>[6x]MGSSWSHPQFEKSSGMNNIDLRVYSFIDSLQPQLASYLATSSQGFLPVPGDACLWIEVAPGMAVHRLSDIALKATNVRLGEQVVERAFGSMEI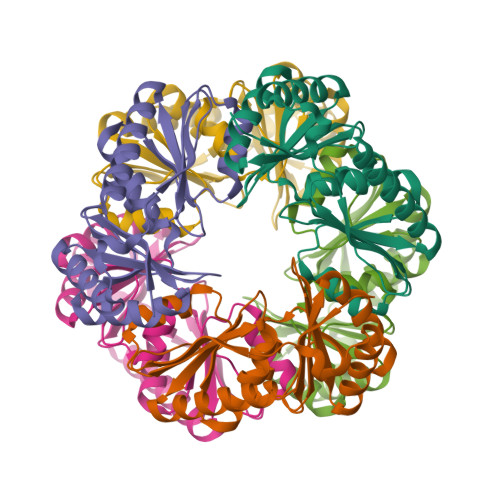HYRNQSDVLASGEAVLREINHAQEDRLPCRIAWKEIIRAITPDHATLINRQLRKGSMLLPGKSMFILETEPAGYIVQAANEAEKAAHVTLIDVRAFGNFGRLTMMGSEAETEEAMRAAEATIASINARARRAEGF> GPSSENKLRQLNLNNEWTLDKLRQRLTKNAQDKLELHLFMLSGIPDTVFDLVELEVLKLELIPDVTIPPSIAQLTGLKELWLYHTAAKIEAPALAFLRENLRALHIKFTDIKEIPLWIYSLKTLEELHLTGNLSAENNRYIVIDGLRELKRLKVLRLKSNLSKLPQVVTDVGVHLQKLSINNE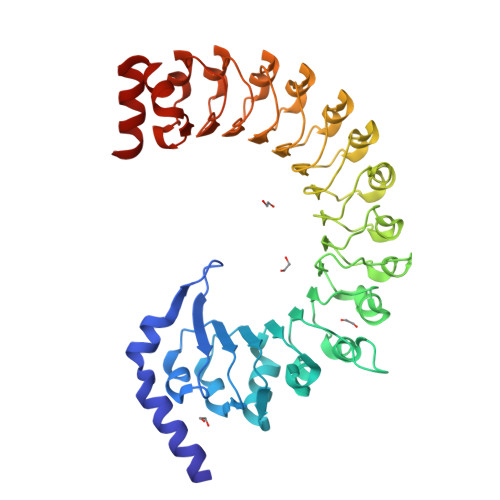GTKLIVLNSLKKMVNLTELELIRCDLERIPHSIFSLHNLQEIDLKDNNLKTIEEIISFQHLHRLTCLKLWYNHIAYIPIQIGNLTNLERLYLNRNKIEKIPTQLFYCRKLRYLDLSHNNLTFLPADIGLLQNLQNLAVTANRIEALPPELFQCRKLRALHLGNNVLQSLPSRVGELTNLTQIELRGNRLECLPVELGECPLLKRSGLVVEEDLFSTLPPEVKERLWRADKEQAA> VSGY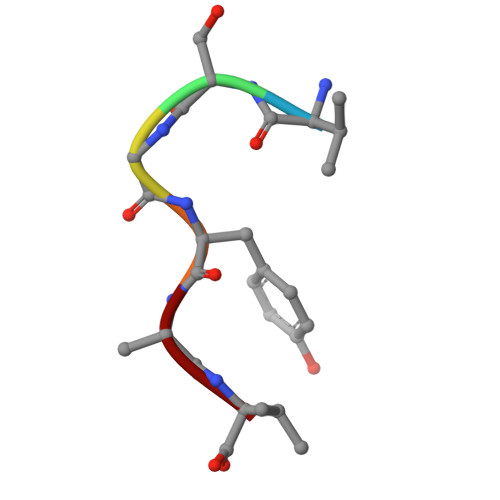AV NS1 is secreted alongside dengue virus particles during an infection. It is a multifunctional protein which exists in different oligomeric forms intracellularly and extracellularly, and they play distinctly different roles. The intracellular NS1 (iNS1), exists as a membrane associated dimeric form and is a part of the viral replication complex. The extracellular secreted NS1 (sNS1), exists in higher oligomeric forms. sNS1 likely causes vascular leakage symptoms in DHF/DSS via two pathways—indirectly, by stimulating the innate immune response through activation of complement and Toll-like receptors, and directly, by binding to endothelial cells causing endothelial hyperpermeability. sNS1 when bound directly to endothelial cells causes barrier dysfunction of the cell monolayer as demonstrated in an in vitro trans-endothelial electrical resistance (TEER) assay. Here we show by cryoEM that the recombinant sNS1 exists in multiple oligomeric states: the tetrameric (stable and loose conformation) and hexameric structures.

We observed two maps that correspond to tetramers: one with clear densities suggesting that the overall structure is quite stable, while the other with looser interactions between the two dimers and poorer map resolution. We refer the former as stable tetramer and the latter as loose tetramer. The difference between the stable and the loose tetramers is whether the residues near the N-terminus form a β-roll or an elongated β-sheet. Hence, this could be the determinant that defines stability. However, we observed loose tetramers forming ~74% of the particle population, while hexamers only form ~3%, suggesting that the loose tetramer may be a preferred oligomerization state. Analysis of the solvent accessibility of the epitopes on the loose tetramer shows two of the epitopes (orange spheres) are partially exposed (37.5%), while the other two (cyan spheres), are fully exposed. Since Fab likely could bind to the loose tetramer and hexamer, this suggests that the loose tetramers and hexamers likely undergo motions that will, at some time point, have their epitopes fully exposed for Fab binding, and once the Fab has bound, the loose tetramer and hexamers could be dismantled into dimers. In conclusion, since the loose tetramer and hexamers are less stable, their quaternary structure can be easily disrupted by antibody binding.

>[4x]HVGCVVSWKNKELKCGSGIFITDNVHTWTEQYKFQPESPSKLASAIQKAHEEGICGIRSVTRLENLMWKQITPELNHILTENEVKLTIMTGDIKGIMQAGKRSLRPQPTELKYSWKAWGKAKMLSTELHNHTFLIDGPETAECPNTNRAWNSLEVEDYGFGVFTTNIWLKLKERQDVFCDSKLMSAAIKDNRAVHADMGYWIESALNDTWKIEKASFIEVKSCHWPKSHTLWSNGVLESEMIIPKNFAGPVSQHNYRPGYHTQTAGPWHLGRLEMDFDFCEGTTVVVTEDCGNRGPSLRTTTASGKLITEWCCRSCTLPPLRYRGEDGCWYGMEIRPLKEK>SGHGMEENGMKSKILIFGGTGYIGNHMVKGSLKLGHPTYVFTRPNSSKTTLLDEFQSLGAIIVKGELDEHEKLVELMKKVDVVISALAFPQILDQFKILEAIKVAGNIKRFLPSDFGVEEDRINALPPFEALIERKRMIRRAIEEANIPYTYVSANCFASYFINYLLRPYDPKDEITVYGTGEAKFAMNYEQDIGLYTIKVATDPRALNRVVIYRPSTNIITQLE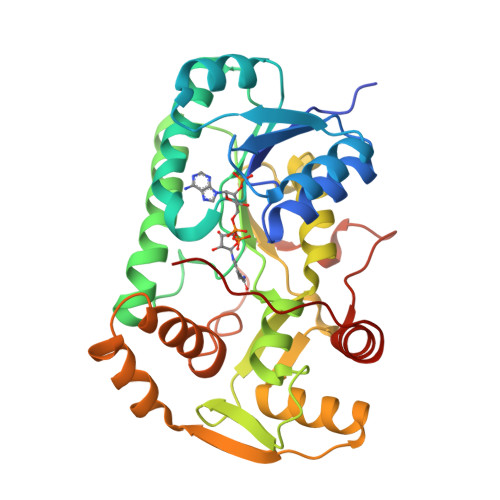LISRWEKKIGKKFKKIHVPEEEIVALTKELPEPENIPIAILHCLFIDGATMSYDFKENDVEASTLYPELKFTTIDELLDIFVHDPPPPASAAF[2x]>MPAAPLDVKCLEANKDYIIISWKQPAVDGGSPILGYFIDKCEVGTDSWSQCNDTPVKFARFPVTGLIEGRSYIFRVRAVNKMGIGFPSRVSEPVAALDPAEKARLKSRPSAPWTGQIIVTEEEPSEGIVPGPPTDLSVTEATRSYVVLSWKPPGQRGHEGIMYFVEKCEAGTENWQRVNTELPVKSPRFALFDLAEGKSYCFRVRCSNSAGVGEPSEATEVTVVGDKLDIP[2x];>GPLGSGILMAPKTFWVNEGKHAKFRCYVMGKPEPEIEWHWEGRPLLPDRRRLMYRDRDGGFVLKVLYCQAKDRGLYVCAARNSAGQTLSAVQLHVKEP[2x]

Obscurin, or its homolog obscurin-like-1, bridges the giant ruler titin and the myosin crosslinker myomesin at the M-band. Myomesin is a 185 kDa modular protein that localizes exclusively at the M-band, where anti-parallel dimers cross link myosin filaments. In addition to a mechanical role, myomesin is also needed for the integration of obscurin and its smaller obscurin-like-1 homolog at the M-band (Fukuzawa et al., 2008). Yeast two-hybrid and biochemical analyses have mapped the obscurin/obscurin-like-1:myomesin interaction to the linker region (L) located between the fourth and fifth Fn-III domains of myomesin (My4 and My5, respectively) and the third Ig domain of either obscurin or obscurin-like-1 (O3 and OL3, respectively) (inset) (Fukuzawa et al., 2008).

Using a matrix microseeding (MMS) approach (D'Arcy et al., 2014), we successfully crystallized the OL3:My4LMy5 complex and solved its structure at the 3.1 Å resolution. While the myomesin My4 domain and its C-terminal linker L as well as obscurin-like-1 OL3 are well defined in the structure, the entire myomesin My5 domain is invisible in electron density maps. The OL3:My4L complex is present as a (OL3:My4L)2 dimer of heterodimers in the crystal. Individual OL3:My4L complexes display a bent dumbbell-shaped structure, in which the myomesin L linker extends away from the My4 domain integrating within the OL3 fold. LH leads the C-terminal portion of L, an 18-amino-acid-long extended stretch divided into two β-strands (LS′ and LS″) that integrate within the OL3 Ig fold. In OL3, the A β-strand that is hydrogen-bonded to B is missing and is replaced by myomesin LS′ (Ser618-Thr622), thus re-establishing a complete Ig architecture. A second myomesin strand (LS″, Ile626-Glu630) also hydrogen bonds to B″ at a position that is reminiscent of the A′ positioning found in a few deviant I-set Ig domains, identified as the I∗-set subtype (Pernigo et al., 2015). Thus, OL3A is a complex trans-complemented hybrid I/I∗-set Ig fold. Overall, the OL3:My4L interface area is 1,046 Å2. In the case of OL3:My4L, this binding mode provides a surprisingly high mechanical stability to the complex (∼135 pN), a rupture force significantly higher than that required to unfold OL3 alone (∼85 pN) and quantitatively similar to that exhibited by the myomesin C-terminal dimer (∼137 pN) (Berkemeier et al., 2011) required for myosin crosslinking.> MVKLNDVLSYVNGLVGKGVDADGWYGTQCMDLTVDVMQRFFGWRPYGNAIALVDQPLPAGFQRIRTTSSTQIKAGDVMIWGLGYYAQYGHTGIATEDGRADGTFVSVDQNW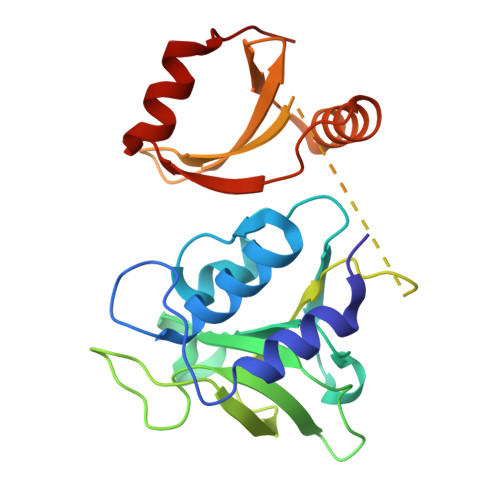INPSLEVGSPAAAIHHNMDGVWGVIRPPYEAASTPKPPAPKPDKPNLGQFKGDDDIMFIYYKRTKQGSTEQWFVIGGKRIYLPTMTYVNEANDLIKRYGGNTNVTTYNHDNFGLKMMEAALPQVKV Here we have determined by cryo-electron microscopy (cryo-EM) structures of the head and tail components of YSD1, a phage infecting Salmonella Typhi. We investigated the structure of the recently characterised phage YSD1 as an example of flagellotropic χ-like phages and more generally phages with long, non-contractile tails. Samples of YSD1 imaged by EM showed characteristic features of siphoviruses: an icosahedral capsid and a flexible tail tube of ~220 nm in length. Cryo-EM analysis of YSD1 allowed structure determination of the head and tail components at resolutions of 3.8 Å and 3.5 Å, respectively, and the generation of de novo models for the major capsid (YSD1_17), auxiliary protein (YSD1_16) and tail-tube protein (YSD1_22).

The 3.5 Å-resolution structure of the YSD1 tail reveals a robust but pliable assembly based on hexameric rings strung around a central spine of the tape measure protein. Our structure of the YSD1 tail reveals that the helical tube is built from hexameric rings of the three-domain tail-tube protein. The rings are stacked with an axial rise of 41.2 Å and a twist of 19.7° to form a right-handed helix. Clear density in the cryo-EM helical reconstruction allowed structure determination of the first two domains. Only weak density is present for the third, C-terminal domain, indicating that it does not strictly follow the helical symmetry of the tail tube. The main body of the tail tube is formed by domain 1, a sandwich composed of two four-stranded β-sheets with a long β-stranded loop extending strands β3 and β4 (β-hairpin). Assembly of the tail tube involves the formation of a continuous antiparallel β-barrel connecting the largest β-sheets of six subunits on the internal face of the tail tube. In the assembled tail, domain 2 stabilises the hexameric ring by wrapping around adjacent subunits and locking them into place like a latch. Unexpectedly, for such an elongated assembly subject to substantial shearing forces, there are relatively few inter-ring interactions. These interactions along the helical axis rely almost exclusively on the extended β-hairpin, which contributes 93% of the inter-ring contact area. The placement of negatively charged aspartate and glutamate residues in the assembled tail tube appears as a right-handed helical track through the tail tube.

>[18x]MNDNYQNNYVVGRGTVYFDRFQDGTNRKTGEMYFGNTPEFTINTDSETLDHYSSDHGMRVMDASVLLEASQGGTFTCDNINADNLALWFLGEVSNTTQTQQTDAKEVFNPIMRGRYYQLGTTDDNPTGVRGVTNFQMVKADASIAISVGSGDITSIVGATVVNPAGNYEIDLEAGRIYIEPDSTDLSGNVQIAVQYDVDAQKRTLVIGKSNMVYGALRMISDNPVGLNKNYYFPKVSIAPDGDYALKGDDWQVMSFTFKAMQLNNITQRVYIDIVEAAAAVDPTAQRTIEITPASTTATTGGAGVVCTVTVRDGTGTAVQGDAVTFTTVAGATVTPNSATTGASGTATTTVNRTAAGTATVTATLANGKAATTGTITFSAP>[9x]SGRFDQYPTKKGDFAIDGYLLDYSSPKQGCWVDGIT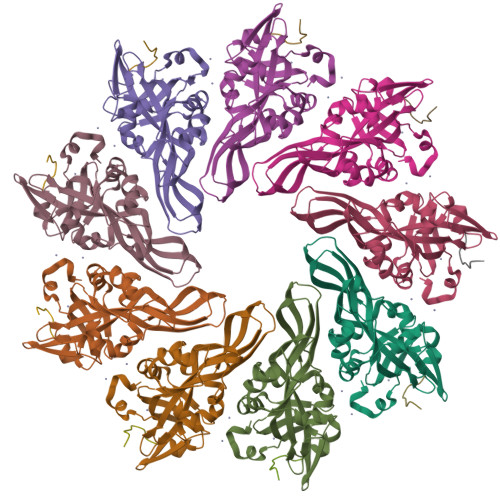VYGDIYIGKQNWGTYTRPVFAYLQYVETISIPQNVTTTLSYQLTKGHTRSFETSVNAKYSVGANIDIVNVGSEISTGFTRSESWSTTQSFTDTTEMKGPGTFVIYQVVLVYAHNATSAGRQNANAFAYSKTQAVGSRVDLYYLSAITQRKRVIVPSSNAVTPLDWDTVQRNVLMENYNPGSNSGHFSFDWSAYNDPHRRY;>QPQSHSIELDEVSKEAASTRAALTSNL[9x]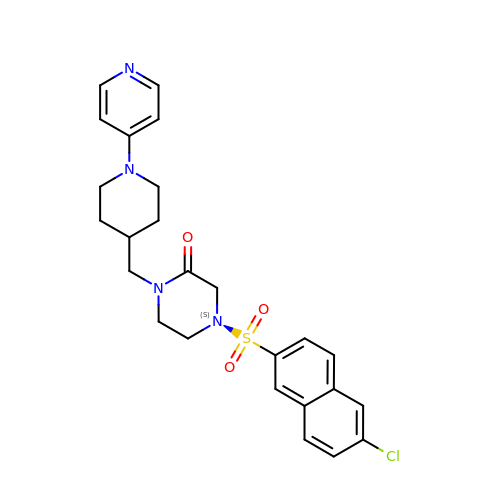4-[(6-CHLORO-2-NAPHTHALENYL)SULFONYL]-1-[[1-(4-PYRIDINYL)-4-PIPERIDINYL]METHYL]PIPERAZINONE | C25 H27 Cl N4 O3 S | BKWIJYNQPXKNMH-UHFFFAOYSA-N>[2x]ATNGKLFPWAQIRLPTAVVPLRYELSLHPNLTSMTFRGSVTISVQALQVTWNIILHSTGHNISRVTFMSAVSSQEKQAEILEYAYHGQIAIVAPEALLAGHNYTLKIEYSANISSSYYGFYGFSYTDESNEKKYFAATQFEPLAARSAFPCFDEPAFKATFIIKIIRDEQYTALSNMPKKSSVVLDDGLVQDEFSESVKMSTYLVAFIVGEMKNLSQDVNGTLVSIYAVPEKIGQVHYALETTVKLLEFFQNYFEIQYPLKKLDLVAIPDFE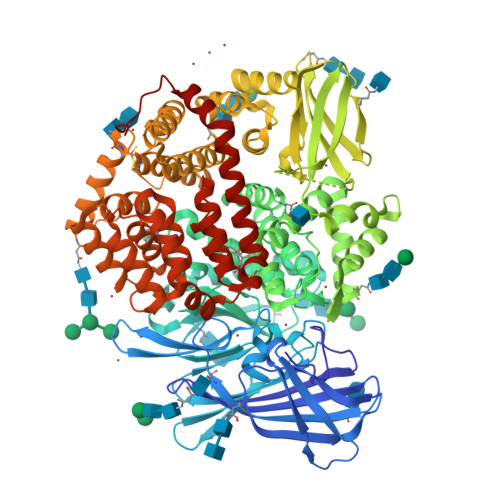AGAMENWGLLTFREETLLYDSNTSSMADRKLVTKIIAHELAHQWFGNLVTMKWWNDLWLNEGFATFMEYFSLEKIFKELSSYEDFLDARFKTMKKDSLNSSHPISSSVQSSEQIEEMFDSLSYFKGSSLLLMLKTYLSEDVFQHAVVLYLHNHSYASIQSDDLWDSFNEVTNQTLDVKRMMKTWTLQKGFPLVTVQKKGKELFIQQERFFLNMKPEIQPSDTSYLWHIPLSYVTEGRNYSKYQSVSLLDKKSGVINLTEEVLWVKVNINMNGYYIVHYADDDWEALIHQLKINPYVLSDKDRANLINNIFELAGLGKVPLKRAFDLINYLGNENHTAPITEALFQTDLIYNLLEKLGYMDLASRLVTRVFKLLQNQIQQQTWTDEGTPSMRELRSALLEFACTHNLGNCSTTAMKLFDDWMASNGTQSLPTDVMTTVFKVGAKTDKGWSFLLGKYISIGSEAEKNKILEALASSEDVRKLYWLMKSSLNGDNFRTQKLSFIIRTVGRHFPGHLLAWDFVKENWNKLVQKFPLGSYTIQNIVAGSTYLFSTKTHLSEVQAFFENQSEATFRLRCVQEALEVIQLNIQWMEKNLKSLTWWLRTETSQVAPA Later, proteins capable of binding and increasing the fluorescent signals of fluorogenic molecules became commonly referred to as fluorogen activating proteins (FAPs). In silico shortlisting with the further screening of the lipocalin Blc mutants launched DiBs FAPs tags family binding green and red BODIPY dyes. It suggests that the easier task of fine-tuning the fluorogen-binding properties of an already functional protein in silico should be readily achievable. To test this hypothesis, we used Rosetta for computational ligand docking followed by protein binding pocket redesign to further improve the previously described FAP DiB1 that is capable of binding to a BODIPY-like dye M739. The designed protein, DiB-RM, shows higher brightness, localization precision, and apparent photostability in protein-PAINT super-resolution imaging compared to its parental variant DiB1.

Moreover, DiB-RM can be cleaved to obtain an efficient split system with enhanced performance compared to a parental DiB-split system. Despite no intentional optimization for it, the DiB-RM-based split protein (DiB-RM-split) created analogously to the previously tested DiB2-split system also behaved better. We have not observed aggregation in the separately expressed N1-109 fragment, and the split protein successfully assembled in living cells without the need of including the additional overlapping β strand in the C fragment. Regardless of lower brightness both in vitro and in super-resolution microscopy set up as well as less stable fluorescent signal compared to full-length DiB-RM tag, we speculate that the DiB-RM-split should be a scaffold of choice for further DiB-split system optimizations.

> MGHHHHHHLESTSLYKKSSSTPPRGVTVVNNFDCKRYLGTWYEIARFDHRAERGLEKVTATYSLRDDGGLNVIFKGYNPDRGMWQQYVGKAYFTGAPTRAALKVAFF;> MGPFYGGYNVIALDREYRHALVCGPDRDYLWINSRTPTISDEVKQEMLAVATREGFDVSKFIWVQQPGS> RPPGFSPF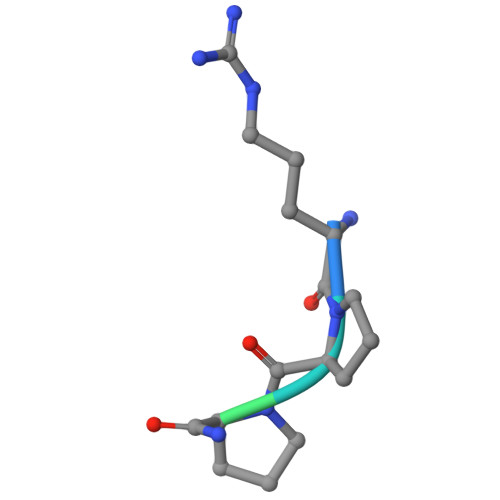R> GHMLEDPKQLAVYEEFARNVPGFLPTNDLSQPTGFLAQPMKQAWATDDVAQIYDKCITELEQHLHAIPPTLAMNPQAQALRSLLEVVVLSRNSRDAIAALGLLQKAVEGLLDATSGADADLLLRYRECHLLVLKALQDGRAYGSPWCNKQITRCLIECRDEYKYNVEAVELLIRNHLVNMQQYDLHLAQSMENGLNYMAVAFAMQLVKILLVDERSVAHVTEADLFHTIETLMRINAHSRGNAPEGLPQLMEVVR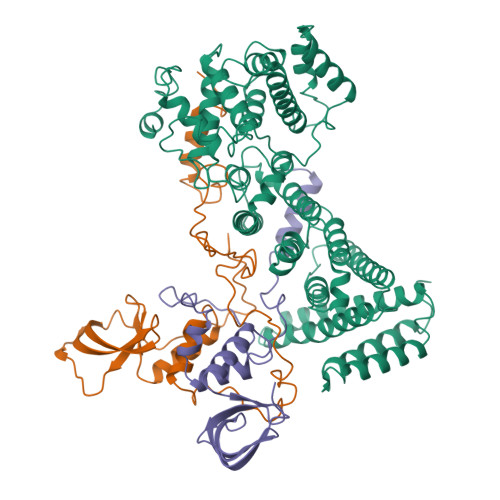SNYEAMIDRAHGGPNFMMHSGISQASEYDDPPGLREKAEYLLREWVNLYHSAAAGRDSTKAFSAFVGQMHQQGILKTDDLITRFFRLCTEMCVEISYRAQAEQQHNPAANPTMIRAKCYHNLDAFVRLIALLVKHSGEATNTVTKINLLNKVLGIVVGVLLQDHDVRQSEFQQLPYHRIFIMLLLELNAPEHVLETINFQTLTAFCNTFHILRPTKAPGFVYAWLELISHRIFIARMLAHTPQQKGWPMYAQLLIDLFKYLAPFLRNVELTKPMQILYKGTLRVLLVLLHDFPEFLCDYHYGFCDVIPPNCIQLRNLILSAFPRNMRLPDPFTPNLKVDMLSEINIAPRILTNFTGVMPPQFKKDLDSYLKTRSPVTFLSDLRSNLQVSNEPGNRYNLQLINALVLYVGTQAIAHIHNKGSTPSMSTITHSAHMDIFQNLAVDLDTEGRYLFLNAIANQLRYPNSHTHYFSCTMLYLFAEANTEAIQEQITRVLLERLIVNRPHPWGLLITFIELIKNPAFKFWNHEFVHCAPEIEKLFQSVAQCCMGQKQAQQVME;> GPHMTNIPQGMVTDQFGMIGLLTFIRAAETDPGMVHLALGSDLTTLGLNLNSPENLYPKFASPWASSPCRPQDIDFHVPSEYLTNIHIRDKLAAIKLGRYGEDLLFYLYYMNGGDVLQLLAAVELFNRDWRYHKEERVWITRAPGMEPTMKTNTYERGTYYFFDCLNWRKVAKEFHLEYDKLEERPHLPSTFNYNPAQQAF;> MGSSHHHHHHSSGTGSGHMLTKEQLYQQAMEEAAWHHMPHPSDSERIRQYLPRNPCPTPPYHHQMPPPHSDTVEFYQRLSTETLFFIFYYLEGTKAQYLAAKALKKQSWRFHTKYMMWFQRHEEPKTITDEFEQGTYIYFDYEKWGQRKKEGFTFEYRYLEDRDLQ> GSHMDFVAFMNKINSINANLSRYENIINQIDAQHKDLLTQVSEEQEMELRRSLDDYISQATDLQYQLKADIKDAQRDGLHDSNKQAQAENCRQKFLKLIQDYRIIDSNYKEESKEQAKRQYTIIQPEATDEEVEAAINDVNGQQIFSQALLNANRRGEAKTALAEVQARHQELLKLEKTMAELTQLFNDMEELVIE;>QGHMSNFLAEQYERDRKAIINCCFSRPDHKTGEPPNNYITHVRIIEDSKFPSSRPPPDSKLENKKKRLLILSAKPNNAKLIQIHKARENSDGSFQIGRTWQLTELVRVEKDLEISEGFILTMSKKYYWETNSAKERTVFIKSLITLYIQTFEGHVPELVNWDLSLFYLDERSYQRAVITNRPGSVSPIKSPTSNFTTNTTQSVGSVPFSAPTERTRRSETESVNPVSTPA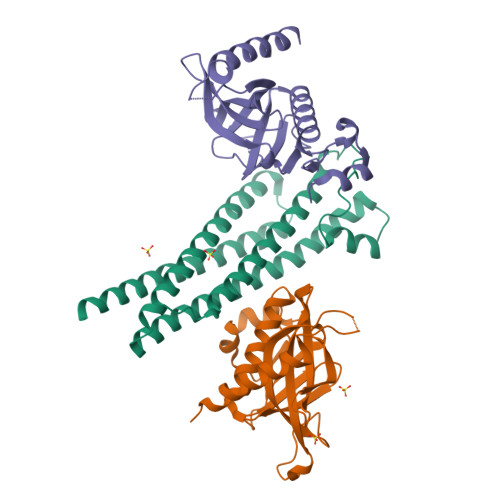SVEYHAGMKSLNKAPYSSNS[2x]> SNAETNEITVGITVTTTGPAAALGIPERNALEFVAKEIGGHPIKMIVLDDGGDPTAATTNARRFVTESKADVIMGSSVTPPTVAVSNVANEAQVPHIALAPLPVTPERAKWSVVMPQPIPIMGKVLYEHMKKNN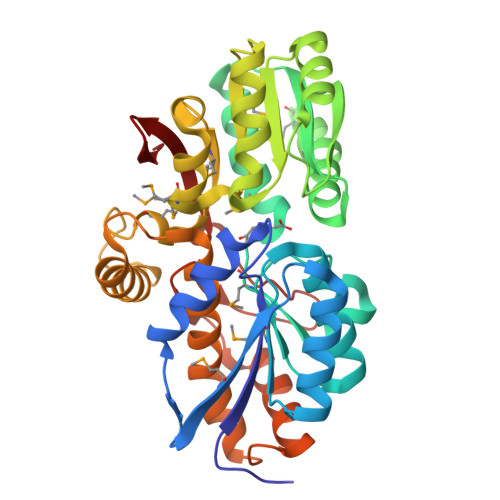IKTVGYIGYSDSYGDLWFNDLKKQGEAMGLKIVAEERFARPDTSVAGQVLKLVAANPDAILVGASGTAAALPQTALRERGYNGLIYQTHGAASMDFIRIAGKSAEGVLMASGPVMDPEGQNDSALTKKPGLELNTAYETKYGPNSRSQFAGHSFDAFKVLERVIPVALKTAKPGTQEFREAIRKALLTEKDIAASQGVYSFTETDRYGLDDRSRILLTVKNGKYVIVK> DCGLPPDVPNAQPALEGRTSFPEDTVITYKCEESFVKIPGEKDSVICLKGSQWSDIEEFCNRSCEVPTRLNSASLKQPYITQNYFPVGTVVEYECRPGYRREPSLSPKLTCLQNLKWSTAVEFCKKKSCPNPGEIRNGQIDVPGGILFGATISFSCNTGYKLFGSTSSFCLISGSSVQWSDPLPECREIYCPAPPQIDNGIIQGERDHYGYRQSVTYACNKGFTMIGEHSIYCTVNNDEGE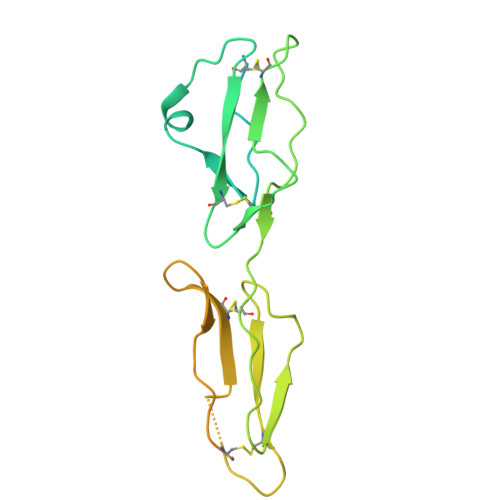WSGPPPECRGHHHHHH> IVGGTSASAGDFPFIVSISRNGGPWCGGSLLNANTVLTAAHCVSGYAQSGFQIRAGSLSRTSGGITSSLSSVRVHPSYSGNNNDLAILKLSTSIPSGGNIGYARLAASGSDPVAGSSATVAGWGATSEGGSSTPVNLLKVTVPIVSRATCRAQYGTSAITNQMFCAGVSSGGKDSCQGDSG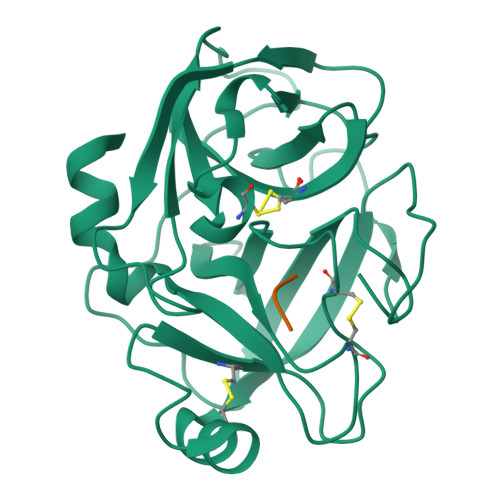GPIVDSSNTLIGAVSWGNGCARPNYSGVYASVGALRSFIDTYA;> GAR>GAMRKIGIIGGTFDPPHYGHLLIANEVYHALNLEEVWFLPNQIPPHKQGRNIT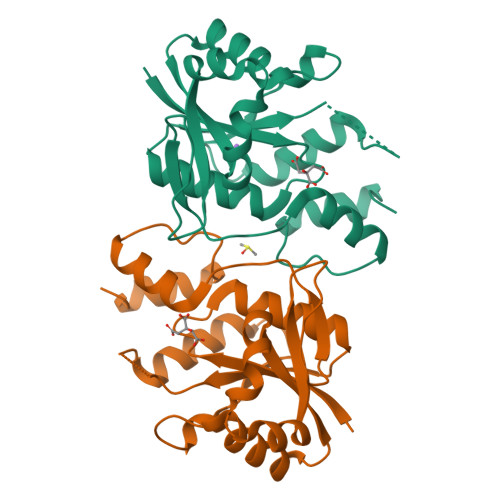SVESRLQMLELATEAEEHFSICLEELSRKGPSYTYDTMLQLTKKYPDVQFHFIIGGDMVEYLPKWYNIEALLDLVTFVGVARPGYKLRTPYPITTVEIPEFAVSSSLLRERYKEKKTCKYLLPEKVQVYIERNGLYES[8x]S-[2-({N-[(2R)-2-hydroxy-3,3-dimethyl-4-(phosphonooxy)butanoyl]-beta-alanyl}amino)ethyl] (5beta,7alpha,8alpha,10alpha,12alpha)-7-hydroxyatis-16-ene-18-thioate | C31 H51 N2 O9 P S | 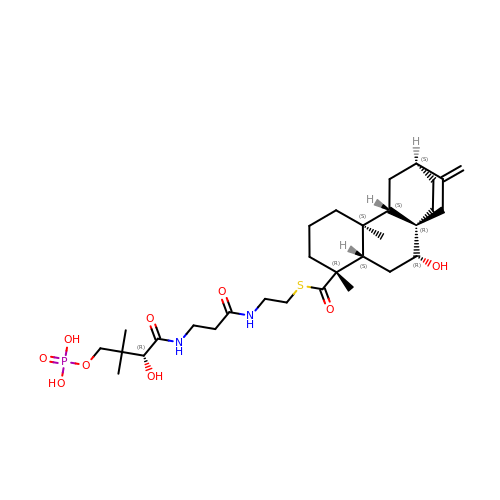PHQDCKXVLPNCFQ-HHFPKWFXSA-N>GANNDMPVEQILEAELAVDPKIDT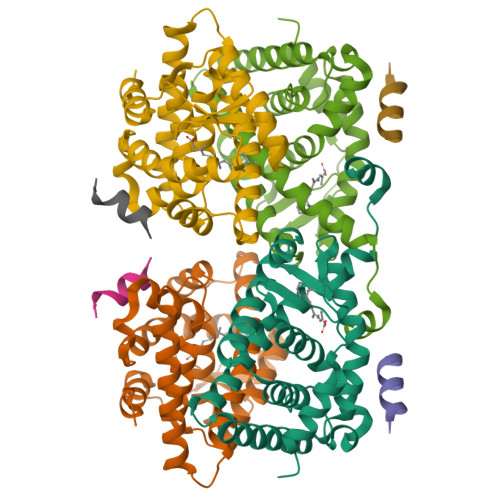YIDAQKDPVTNICQAADKQLFTLVEWAKRIPHFTELPLEDQVILLRAGWNELLIAGFSHRSIMAKDGILLATGLHVHRSSAHQAGVGTIFDRVLTELVAKMRDMKMDKTELGCLRAVVLFNPDAKGLTAVQEVEQLREKVYASLEEYTKSRYPEEPGRFAKLLLRLPALRSIGLKCLEHLFFFKLIGDQPIDTFLMEMLENPSPAT[2x];>[2x]RHKILHRLLQEGSPS> KVTMNDFDYLKLLGKGTFGKVILVREKATGRYYAMKILRKEVIIAKDEVAHTVTESRVLQNTRHPFLTALKYAFQTHDRLCFVMEYANGGELFFHLSRERVFTEERARFYGAEIVSALEYLHSRDVVYRDIKLENLMLDKDGHIKITDFGLCKEGISDGATMKTFCGTPEYLAPEVLEDNDYGRAVDWWGLGVVMYEMMCGRLPFYNQDHERLFELILMEEIRFPRTLSPEAKSLLAGLLKKDPKQRLGGGPSDAKEVMEHRFFLSI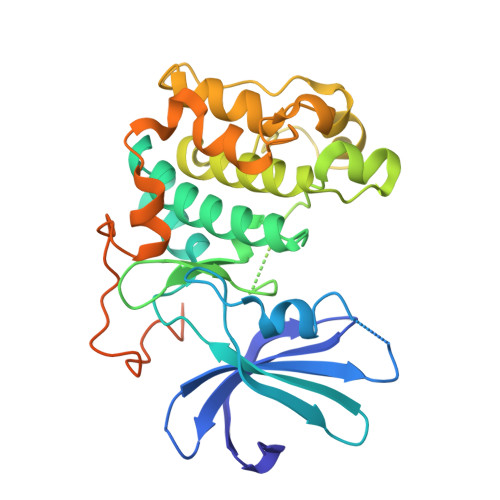NWQDVVQKKLLPPFKPQVTSEVDTRYFDDEFTAQSITITPPDRYDSLGLLELDQRTHFPQFSYSASIR10-(4-hydroxyphenyl)-2,4-dioxo-2,3,4,10-tetrahydropyrimido[4,5-b]quinoline-8-carbonitrile 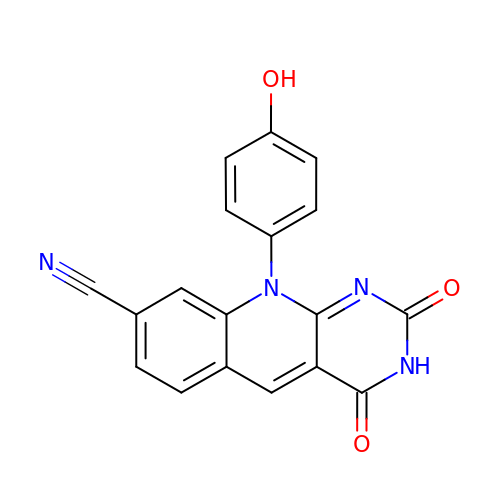| C18 H10 N4 O3 | JAOMIQIQBBRLQX-UHFFFAOYSA-N O-SULFO-L-TYROSINE | C9 H11 N O6 S | 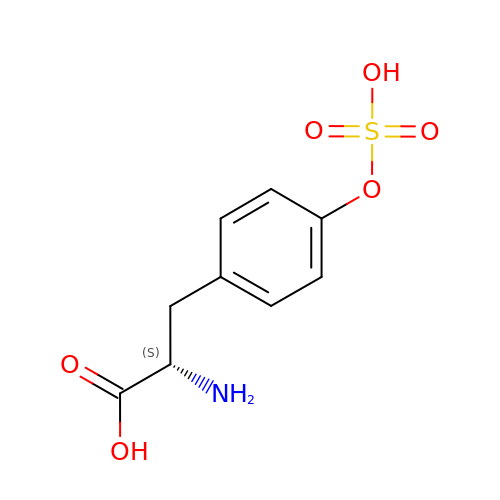CIQHWLTYGMYQQR-QMMMGPOBSA-N(1-ethylpyrazol-4-yl)methyl 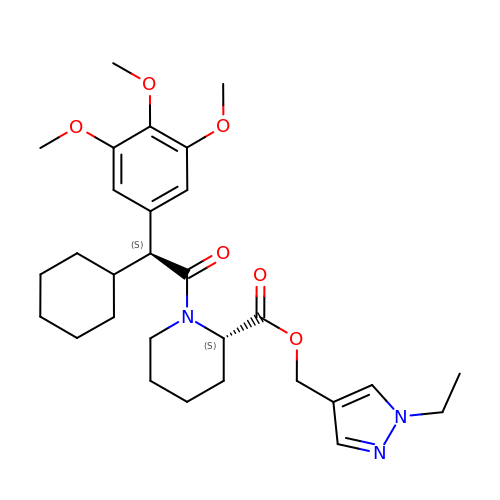(2S)-1-[(2S)-2-cyclohexyl-2-(3,4,5-trimethoxyphenyl)ethanoyl]piperidine-2-carboxylate | C29 H41 N3 O6 | SLRMGPGDBBZIPB-OZXSUGGESA-N spiro[1H-2-benzofuran-3,4'-piperidine] | C12 H15 N O | 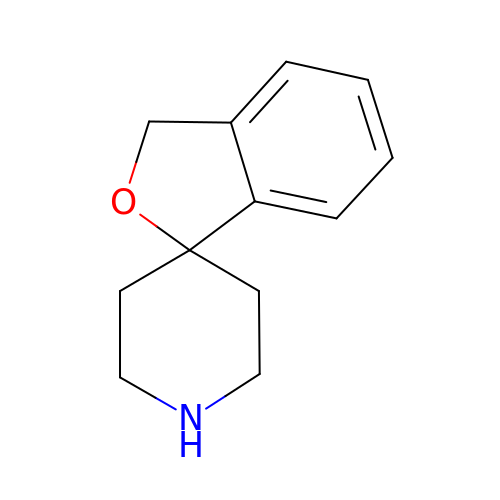BYOIMOJOKVUNTP-UHFFFAOYSA-N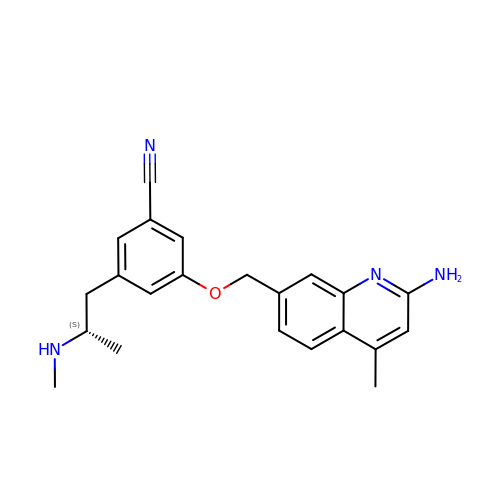3-[(2-amino-4-methylquinolin-7-yl)methoxy]-5-[(2S)-2-(methylamino)propyl]benzonitrile | C22 H24 N4 O | PUGNZMCPLRURSU-HNNXBMFYSA-N>[2x]GSHMGGGGGIVLFVDFDYFYAQVEEVLNPSLKGKPVVVCVFSGRFEDSGAVATANYEARKFGVKAGIPIVEAKKILPNAVYLPMRKEVYQQVSSRIMNLLREYSEKIEIASIDEAYLDISDKVRDYREAYNLGLEIKNKILEKEKITVTVGISKNKVFAKIAADMAKPNGIKVIDDEEVKRLIRELDIADVPGIGNITAEKLKKLGINKLVDTLSIEFDKLKGMIGEAKAKYLISLARDEYNEPIRTRVRKSIGRIVTMKRNSRNLEEIKPYLFRAIEESYYKLDKRIPKAIHVVAVTEDLDIVSRGRTFPHGISKETAYSESVKLLQKILEEDERKIRRIGVRFSKFIEAIGLDKFFDT

Y-family polymerases are able to bypass a variety of DNA lesions that impede high-fidelity replicative DNA polymerases. 7,8-dihydro-8-oxoguanine (oxoG) is the major known product of oxidation of DNA by reactive oxygen species induced by either ionizing radiation, photochemical mechanisms, or normal cellular metabolic activity. Our kinetic primer extension studies demonstrate that the bypass polymerase Dpo4 preferentially inserts C opposite oxoG, and also preferentially extends from the oxoG•C base pair, thus achieving error-free bypass of this lesion. The Dpo4 polymerase embraces the 19-mer template/13-mer primer DNA by its four domains: palm (residues 1–10 and 78–166), finger (residues 11–77), thumb (residues 167–233), and little-finger (residues 244–341).

In the case of the postinsertion binary complex, a covalently incorporated cytosine is positioned opposite the oxoG site and forms a Watson-Crick oxoG•C pair. Residues 3–19 of the template strand can be traced in the electron density map. The finger domain is positioned directly over the Watson-Crick oxoG•C pair with one Ca2+ cation coordinated by the D7, D105, and E106 at the active site of Dpo4. Upon covalent cytosine incorporation, there is retention of little-finger contacts with the phosphate groups of C7, T8, A9, and C10 on the template strand, and the phosphate groups of G6, A7, and T8 on the primer strand. By contrast, the contact of the thumb domain with the phosphate group of T13 is relocated to the phosphate group of A12 on the template strand. At the same time, related thumb-domain contacts on the primer strand are displaced from the phosphate groups of T11 and A12 to the phosphate groups of A12 and G13. Upon covalent base incorporation, the restoration of the B-DNA conformation between the nascent base pair and its adjacent base pair propagates toward the 5′ end of the primer strand. The conformational transition accompanying a restoration of the B-DNA step results in the contacts between the α-helical segments of the thumb domain and DNA phosphate backbone shifting by one step.> RTAAYVALAAASAEAFSTPALSGLKMAEPAQISRKDVLTTAAGAAIIAMPTLAGAASLDPKTGFPIQGGSREKLCGGSASAGCQPMTQAASILDKQRTVLAGKITVAANKVPVLTAAVDKMKTAKKPKLDRDYVLRYSALYLTTLVDAMEQYCLRDANGAKAAGGAGLPKFKETLKPASSSSLYSYVDTVKSGIAAVSAAAKAGDFDGVNKAAGDIKTAADSFLSTANPPIIFN

Photosynthetic cryptophytes are eukaryotic algae that utilize membrane-embedded chlorophyll a/c binding proteins (CACs) and lumen-localized phycobiliproteins (PBPs) as their light-harvesting antennae. Here, we solved four structures of cryptophyte PSI-CAC complexes purified from Rhodomonas salina (Rs) cells grown at L- and S-phase. The R. salina cells grown for six and 12 days (corresponding to L-phase and S-phase) were harvested, and utilized to isolate PSI-CAC complexes. We then solved four structures of PSI-CAC complexes purified from cells in both growth phases, containing either 14 or 11 CACs, and termed them as PSI-14CACL-phase and PSI-11CACL-phase for L-phase models, and PSI-14CACS-phase and PSI-11CACS-phase for S-phase models. Comparison of the four structures reveals how cryptophytes adjust their PSI antennae in response to the different growth state.

Local refinement targeting the PsaQ in PSI-14CACL-phase was performed, resulting in a final local map with the resolution of 3.5 Å. Based on our high-quality cryo-EM map and transcriptome sequencing results, we determined the identity of the lumen-localized protein, which is an uncharacterized yet highly conserved protein in cryptophytes. The overall folding of this protein is similar to the PSII extrinsic subunit PsbQ. PsaQ contains four helices and harbors two chlorophyll molecules. One chlorophyll (Chl a323) is coordinated by the C-terminal residue N234, while the other (Chl a322) is presumably coordinated by a water molecule. PsaQ possesses a long loop between helix 2 and 3 (2/3-loop) which, together with the two chlorophylls, inserts into the membrane plane at the interfacial region between CAC-i and PsaB. Moreover, the N-terminal fragment of PsaQ fills in the gap between CAC-i and CAC-h. Multiple hydrogen bond interactions between PsaQ and CAC-i/PsaB tether the PsaQ protein to the lumen surface of thylakoid membrane. Our structure showed that Chls a322/a323 of PsaQ are in close proximity to Chls a616/a606 in CAC-i and Chl a816 in PsaB. PsaQ is unique to cryptophytes and the chlorophyll-coordinating residue N234 is extremely conserved in PsaQ homologs, suggesting that PsaQ and the bound chlorophylls are crucial for the proper functioning of cryptophyte cells during L-phase.The pathogenic bacterium Shigella flexneri uses a type III secretion system to inject virulence factors from the bacterial cytosol directly into host cells. One of the inner membrane components, Spa40, belongs to a family of proteins proposed to regulate the switching of substrate specificity of the export apparatus. The S. flexneri protein Spa40 has been identified as a component of the basal body and is predicted to have a large, N-terminal transmembrane domain (Spa40TM) and a C-terminal cytoplasmic domain (Spa40C). In summary, we have shown that the S. flexneri homologue of the T3SS substrate switching protein, Spa40, is cleaved on the N-terminal side of P258 within the highly conserved NPTH sequence to produce a stable complex consisting of the subdomains, Spa40CN and Spa40CC.

The model comprises residues 237–257 of Spa40CN (residues 207–236 were present in the construct but not visible in electron density) and 258–338 of Spa40CC (the last four residues, 339–342, were not visible in electron density). The structure was refined using data to 2 Å with residuals Rwork and Rfree of 17.8% and 22.7% respectively. The structure of Spa40C consists of a central β-sheet surrounded by four α-helices. The structured region of Spa40CN consists of a single α-helix (α1) followed by a single β-strand (β1) that lies at the centre of the structure and forms one strand of the five-stranded β-sheet. The structure of Spa40CC starts at P258 and consists of four β-strands and three α-helices that wrap around β1 of Spa40CN. The NPTH sequence lies on a loop between β1 and β2, the PTH region having flipped away from N257, revealing that the cleavage of the N257-P258 peptide bond results in a conformational change to this loop region. P258 moves ∼10 Å from the catalytic asparagine residue and both P258 and T259 are less well-ordered than the surrounding residues, as indicated by higher isotropic temperature factors. The striking feature of these structures is that Spa40CN forms part of the core of the fold with the conserved hydrophobic residues L253 to M256 (LVVM) completely buried by the surrounding Spa40CC structure. In Spa40, the face of this helix that is exposed on the surface is composed of residues K305, R308, K309 and K312, resulting in a highly positively charged patch. In our structure of Spa40, we observe a C-terminal helix of equivalent length to that of EscU.

> MDMMMDKQEIKREYIEQEGHFETKSRRRELHIEILSEQTKSDIRNSKLVVMN;> PTHIAIGIYFNPEIAPAPFISLIETNQCALAVRKYANEVGIPTVRDVKLARKLYKTHTKYSFVDFEHLDEVLRLIVWLEQVENTHLEHHHHHH Strigolactones (SLs) play fundamental roles in regulating plant architecture, which is a major factor determining crop yield. The perception and signal transduction of SLs require the formation of a complex containing the receptor DWARF14 (D14), an F-box protein D3 and a transcriptional regulator D53 in an SL-dependent manner. When the SL level is low, D53 interacts with the transcriptional repressor TOPLESS through its EAR motif and inhibits downstream gene expression. D53 belongs to the AAA+ ATPase family and comprises four distinct domains: the N-terminal region, the D1 ATPase domain, the bridge M domain and the D2 ATPase domain.

Here, we found that apo-D53 was rather flexible and reconstituted the holo-complex containing D53, S-phase kinase-associated protein 1 (SKP1), D3 and D14 with rac-GR24. The cryo-electron microscopy (cryo-EM) structure of SKP1−D3−D14 in the presence of D53 was analyzed and superimposed on the crystal structure of ASK1−D3−AtD14 without D53. After 3D classification, a subset of 42,499 particles remained and was used for reconstruction, yielding a final cryo-EM map with a resolution of 7.09Å estimated by the gold Fourier shell correlation standard. D14, D3 and SKP1 had good fits to the refined map. Unfortunately, front, tilted and side views of the cryo-EM map did not reveal the location of D53. Unfortunately, D53 was too flexible to capture in a certain form, and the electron density information was lost during average and classification processing. No large conformational rearrangement was observed between the structures of the two complexes. Compared with the ASK1−D3−AtD14 complex, D14 in the SKP1−D3−D14 complex was flipped away from D3 at ∼9Å. Although the density does not have enough details to allow for accurate fitting of the SKP1−D3−D14 structure and the approximate 9Å rotation may relate to the difference in D14 proteins from rice and Arabidopsis, the local conformational differences are still possibly associated with the formation of holo-complex. The protected regions of D14 and D3 mainly lie around the interfaces of D14 and D3 in the SKP1−D3−D14 complex, suggesting that D53 may also bind the interfaces of D14 and D3 in a manner dependent on the SL-induced D14−D3 assembly.

> MAEEEEVEEGRSSSSAILDLPEPLLLHILSFLTDVRSRHRAALACGRMRAAERATRSELSLRGDPRSPGFLFLSHAFRFPALEHLDLSLVSPWGHPLLSSVPPCGGGGGGAPSASSSSGMNVYHPEAISEQNAFIAARLAGCFPAVTSLAVYCRDPTTLANLTPHWQASLRRVKLVRWHQRPPTLPDGADLEPLLETCAALRELDLSEFYCWTEDVVRALTTHPSATAALTHLDLGLAAATDGFKSSELGPIAASCPNLRKLVAPCLFNPRFSDCVGDDALLSLATSCPRLTVLRLSEPFEAAANIQREEAAITVAGLVAFFAALPALEDFTMDLQHNVLEAAPAMEALARRCPRIKFLTLGSFQGLCKASWLHLDGVAVCGGLESLYMKNCQDLTDASLAAIGRGCRRLAKFGIHGCDLVTSAGIRRLAFTLRPTLKEVTVLHCRLLHTAECLTALSPIRDRIESLEINCVWNTTEQPCSVANGTTTECDPEDDELGEVYESAAKKCRYMEFDDLGSWEMLRSLSLWFSAGQLLSPLISAGLDSCPVLEEISIKVEGDCRTCPRPAPRTIFGLSDLAGFPVLAKMKLDLSEAVGYALTAPTGQMDLSLWERFYLHGIESLQTLYELDYWPPQDKDVHHRSLTLPAVGLIQRCVGLRKLFIHGTTHEHFMTFFLSIPNLRDMQLREDYYPAPENDLMFTEMRAESWLRFEVQLNSRQIDD;> MAAEAETKAMITLRSCEGQVFEVAEAVAMESQTIRHMIEDKCADTGIPLPNVSAKILSKVIEYCSKHVEARGGAAAAADGDAPAPAAVEANKAVEDELKTFDAEFVKVDQSTLFDLILAANYLNIKGLLDLTCQTVADMIKGKTPEEIRKTFNIKNDFTPEEEEEVRRENQWAFE;> MLRSTHPPPSSPSSSSSGGGGGGGSSASSSSEKTMVGGGGGGGGGSGSAAPSGAKLLQILNVRVVGSGERVVVLSHGFGTDQSAWSRVLPYLTRDHRVVLYDLVCAGSVNPDHFDFRRYDNLDAYVDDLLAILDALRIPRCAFVGHSVSAMIGILASIRRPDLFAKLVLIGASPRFLNDSDYHGGFELEEIQQVFDAMGANYSAWATGYAPLAVGADVPAAVQEFSRTLFNMRPDISLHVCQTVFKTDLRGVLGMVRAPCVVVQTTRDVSVPASVAAYLKAHLGGRTTVEFLQTEGHLPHLSAPSLLAQVLRRALARY>[2x]MHTKKDKKVISLQERVENAVDVSGAFDNCFFHNFALYLLTNNLPLPDDLFHFKSIINRNSKAEQLFEFFHNPESLNLFSILDKENDVSEPSGYLFEKSLILGFLLREWFPTQLVNNSAVKAEMLE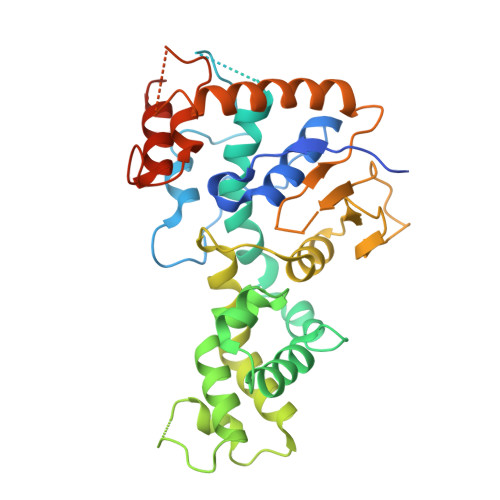GEKGVFSAFKNYKEYRSFMSKEELKSTEFGALYEANEAFLEYFYNRSESTLINKDSPFEKYFVGSSSDEEAIKNYWDAEGYTLYCQHLAKPQVKLSYIEIMTMMKVINQPLTIYDRSTSSIVAEYVNPKVNLPDFEVAIDALQGHYFLLKTEETEKELEEYERSYAQYKRDRSEILAHSDKPVSSLLVRATCPKGHLDEDPFIALIESLSEINSLSQIDTNLKNENT>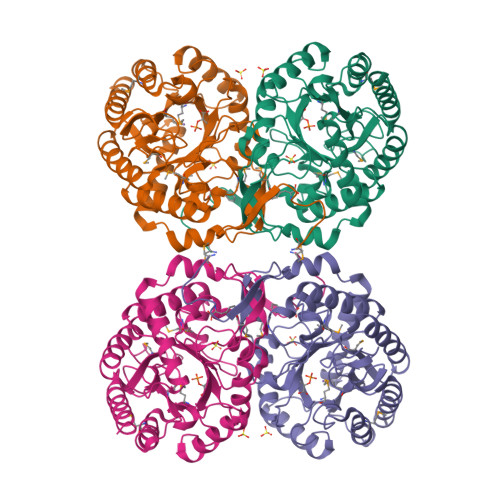[8x]MNYQNDDLRIKEIKELLPPVALLEKFPATENAANTVAHARKAIHKILKGNDDRLLVVIGPCSIHDPVAAKEYATRLLALREELKDELEIVMRVYFEKPRTTVGWKGLINDPHMDNSFQINDGLRIARKLLLDINDSGLPAAGEFLDMITPQYLADLMSWGAIGARTTESQVHRELASGLSCPVGFKNGTDGTIKVAIDAINAAGAPHCFLSVTKWGHSAIVNTSGNGDCHIILRGGKEPNYSAKHVAEVKEGLNKAGLPAQVMIDFSHANSSKQFKKQMDVCADVCQQIAGGEKAIIGVMVESHLVEGNQSLESGEPLAYGKSITDACIGWEDTDALLRQLANAVKARRG> GAAEAGITGTWYNQLGSTFIVTAGADGALTGTYESAVGNAESRYVLTGRYDSAPATDGSGTALGWTVAWKNNYRNAHSATTWSGQYVGGAEARINTQWLLT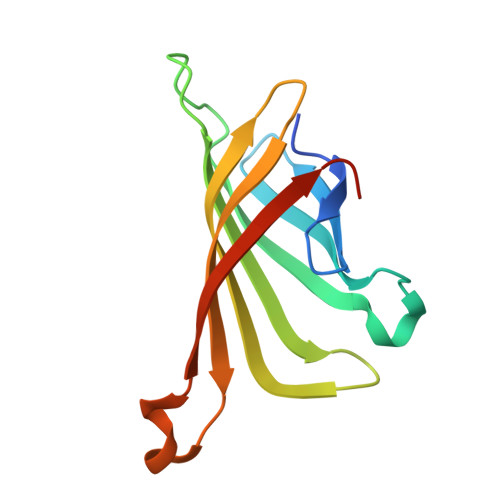SGTTEANAWKSTLVGHDTFTKVKPSAAS> MPYYAFAEPFFIHAITHLHVGSGSSVEEEIDLPFQRDELGYPTIYASSLKGAIKSFLLKEFPDKRDVIYKVLGEDENPEEASLGTFLDAILFAIPSRIIEIDSAKPYVWVYVTTYELLKKVKLYLDSISQLSNASFSNLKNKID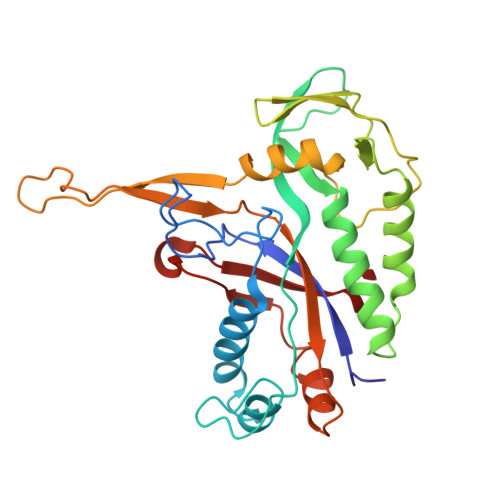TILAKEGKNITLDSDLKSAILNEDFYVELEALNNKIPSIINAGVPLLVLEDSIGREVINRSLIRVRRIRIDRDKKVVETGGLWSEEYVPMKTIFFSVLLGKESKESAIFASCILRNLRYVILGGKETIGKGIVELRWVKDVI(2~{E})-5,6-dimethoxy-2-[[1-(phenylmethyl)piperidin-4-yl]methylidene]-3~{H}-inden-1-one | C24 H27 N O3 | 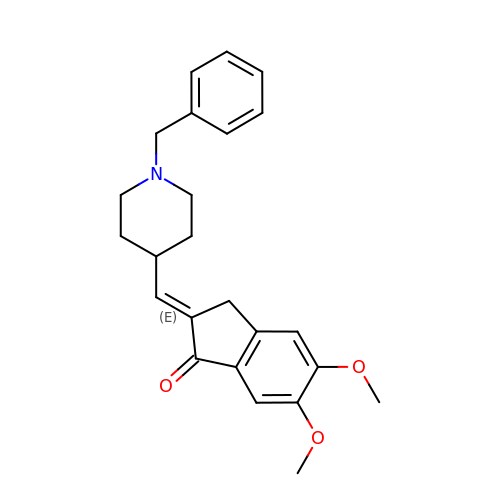LPMOTUSFDTTWJL-UDWIEESQSA-N> GSHMGVEEPVYDATGKPLFGDPSEVHPQSTLKLPHDRGRGNIKTTLKNLPRKGDCRSGNHLGPVSGIYVKPGPVFYQDYMGPVYHRAPLEFFSEAQFCEVTKRIGRVTGSDGRLYHIYVCIDGCILLKLAKRGEPRTLKWIRNFTDCPLWVTSC

Pestiviruses, such as bovine viral diarrhea virus (BVDV) and classical swine fever virus (CSFV) use a virally encoded protein, the N-terminal protease (Npro), to suppress the transcriptional activation of the IFN-α/β genes by interacting with IRF3 and inducing its ubiquitination and proteasome-dependent degradation. The Npro protein is a leader cysteine autoprotease that cleaves itself from the nascent polyprotein during translation of the viral mRNA, freeing itself for innate immune suppression activities. Npro has a unique ‘clam shell’-like protease fold that is distinct from other known proteins including all known proteases. As predicted, Npro consists of two domains, a cysteine protease domain and a zinc-binding domain.

Here, we report the crystal structures of CSFV Npro and a C168A cleavage site Npro mutant to 1.6 Å resolution. The first 19 amino acids are not essential for proteolytic activity of Npro and can be deleted without affecting the in vitro protease activity. The structures presented here show that the C-terminal β-strand (one half of the product peptide) remains buried in the active site pocket, indicating that once cleaved, the C-terminus of Npro acts as an intramolecular inhibitor and thus prevents trans-activity, i.e, the enzyme is inactive toward additional substrates. Additionally, the short α-helix containing the catalytic Cys69 is disordered in the wild-type Npro structure, which may be an additional measure to deactivate the protease function after initial cleavage. In comparison, CSFV Npro structures do not have a disulfide bond between Cys69 and Cys168 because the active site-containing helix is disordered in the wild-type Npro and Cys168 is replaced in the C168A Npro. Thus, the CSFV Npro structure supports the classical cysteine protease mechanism rather than the catalytic mechanism proposed for BVDV Npro.> SANTNHQYAVIAYFYGNASLQGANATINIWEPNLKNPNGDFSLTQIWISAGSGSSLNTIEAGWQVYPGRTGDSQPRFFIYWTADGYTSTGCYDLTCPGFVQTNNYYAIGMALQPSVYGGQQYELNESIQRDPATGNWWLYLWGTVVGYWPASIYNSITNGADTVEWGGEIYDSSGTGGFHTTTQMGSGHFPTEGYGKASYVRDLQCVDTYGNVIS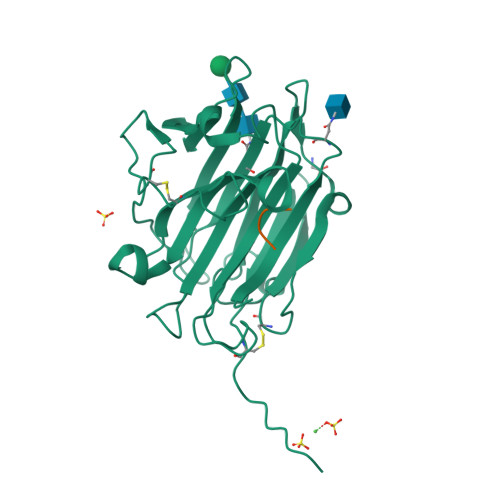PTANSFQGIAPAPNCYNYQFQQGSSELYLFYGGPGCQAIAHHHHHH;> GGGG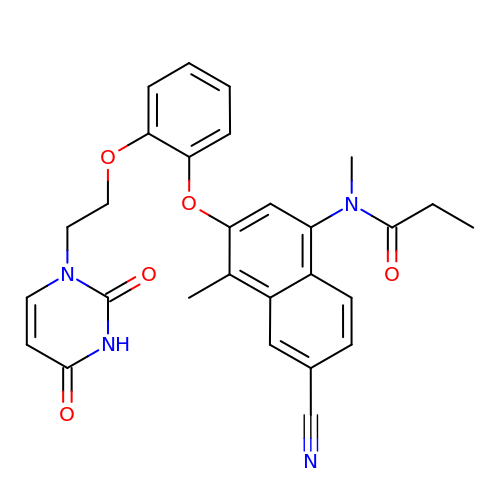N-(6-cyano-3-{2-[2-(2,4-dioxo-3,4-dihydropyrimidin-1(2H)-yl)ethoxy]phenoxy}-4-methylnaphthalen-1-yl)-N-methylpropanamide | C28 H26 N4 O5 | PCQZQAHLCHIVOG-UHFFFAOYSA-N MERTK is a member of the TAM (TYRO3, AXL, and MERTK) receptor tyrosine kinase family. Myeloid epithelial reproductive proto-oncogene tyrosine kinase (MERTK) plays an essential role in modulating cancer immune tolerance by regulating macrophage efferocytosis. MERTK is activated by autophosphorylation when protein S or growth arrest-specific 6 (GAS6) ligands that bind to phosphatidylserine (PtdSer) are exposed on the surface of dying or dead cells bind to MERTK. Therefore, the active/inactive state of kinases can be determined by DFG and αC conformation: the active conformation of kinases should adopt the “DFG flip-in” and “αC swing-in” conformation; all other conformations in DFG and αC are inactive kinases.

Previously, a thermal shift assay using purified MERTK kinase domains in an in-house kinase-inhibitor library revealed that 8 of 356 compounds exhibited a melting temperature shift of >1 °C15. Among them, BMS794833 (IUPAC name; N-[4-(2-amino-3-chloropyridin-4-yl)oxy-3-fluorophenyl]-5-(4-fluorophenyl)-4-oxo-1H-pyridine-3-carboxamide; Fig. 1a), which is currently being studied in phase I clinical trial as a treatment for advanced solid tumors, was co-crystallized with the MERTK kinase domain. The X-ray crystal structure was determined at a resolution of 2.16 Å. The clear electron density map for BMS794833 showed that it occupied both the ATP-binding pocket and the allosteric back pocket (also called the hydrophobic patch). BMS794833 formed two H bonds with the ATP-binding site and two H bonds with the allosteric back pocket of MERTK. The amine and imine at the 3-chloropyridin of BMS794833 formed H bonds with the main chain of Met674 of the ATP-binding site. Two oxygens in the 4-oxo-1,4-dihydropyridine-3-carboxamide group of BMS794833 formed H bonds with the side chain of Lys619 and the main chain amine of Asp741. Specifically, 3-chloropyridine-2-amine interacts with Ala617, 1-fluoro-2-methoxybenzene interacts with Leu671 (gatekeeper) and Phe742, and fluorobenzene interacts with Ile650, Asp741, and Phe719. No salt bridge was formed between Lys619 at the β3 strand and Glu637 at the αC, which is essential for the active conformation, and the αC-helix extended outward from the ATP-binding site. BMS794833 is a typical type II inhibitor with a DFG-out and αC-out conformation, with a similar binding mode to MERTK as LDC1267 but similar to merestinib in its chemical structure.

> GSHMEELQNKLEDVVIDRNLLILGRILGEGEFGSVMEGNLKQEDGTSLKVAVKTMKLDNSSQREIEEFLSEAACMKDFSHPNVIRLLGVCIEMSSQGIPKPMVILPFMKYGDLHTYLLYSRLETGPRHIPLQTLLRFMVDIALGMEYLSNRNFLHRDLAARNCMLRDDMTVCVADFGLSKKIYSGDYYRQGRIAKMPVKWIAIESLADRVYTSKSDVWAFGVTMWEIATRGMTPYPGVQNHEMYDYLLHGHRLKQPEDCLDELYEIMYSCWRTDPLDRPTFSVLRLQLERLLESLPDV> AEYVRALFDFNGNDEEDLPFKKGDILRIRDKPEEQWWNAEDSEGKRGMI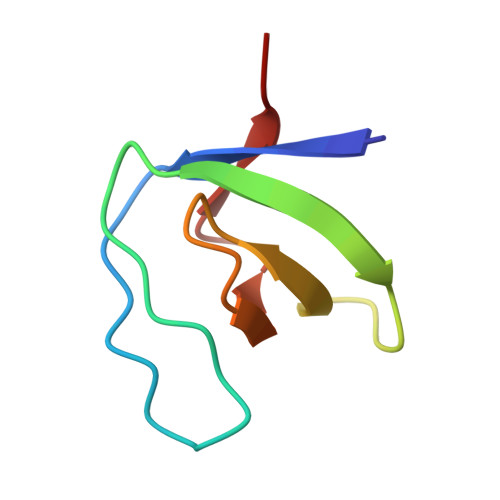PVPYVEKYR RESVERATROL 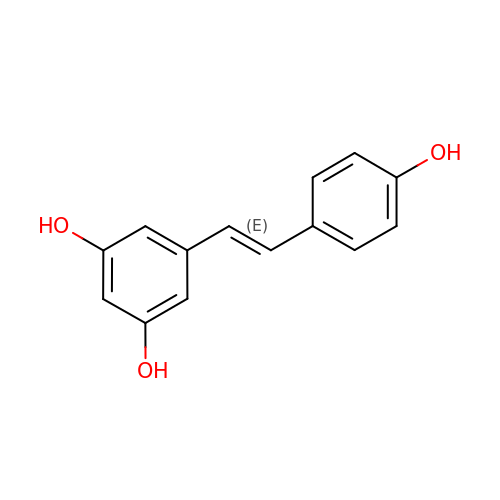| C14 H12 O3 | LUKBXSAWLPMMSZ-OWOJBTEDSA-N> SHMGIFSYKDLDENASKALFSDALAISTYAYHNIDNGFDEGYHQTGFGLGLPLTLITALIGSTQSQGGLPGLPWNPDSEQAAQEAVNNAGWSVISATQLGYAGKTDARGTYYGETAGYTTAQAEVLGKYDSE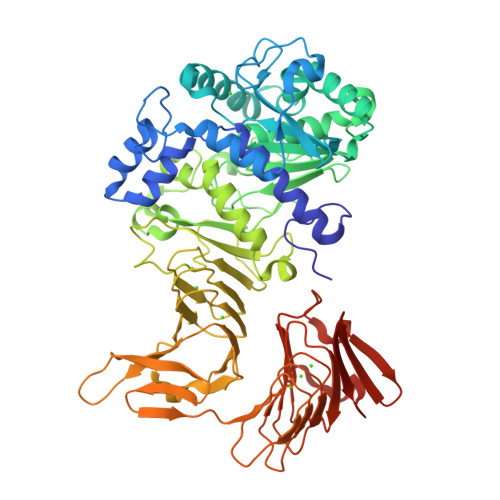GNLTAIGISFRGTSGPRESLIGDTIGDVINDLLAGFGPKGYADGYTLKAFGNLLGDVAKFAQAHGLSGEDVVVSGHSLGGLAVNSMAAQSDANWGGFYAQSNYVAFASPTQYEAGGKVINIGYENDPVFRALDGTSLTLPSLGVHDAPHTSATNNIVNFNDHYASDAWNLLPFSILNIPTWLSHLPFFYQDGLMRVLNSEFYSLTDKDSTIIVSNLSNVTRGNTWVEDLNRNAETHSGPTFIIGSDGNDLIKGGKGNDYLEGRDGDDIFRDAGGYNLIAGGKGHNIFDTQQALKNTEVAYDGNTLYLRDAKGGITLADDISTLRSKETSWLIFNKEVDHQVTAAGLKSDSGLKAYAAATGGDGDDVLQARSHDAWLFGNAGNDTLIGHAGGNLTFVGGSGDDILKGVGNGNTFLFSGDFGRDQLYGFNASDKLVFIGTEGASGNIRDYATQQNDDLVLAFGHSQVTLIGVSLDHISTDQVVLA SELENATE ION | O4 Se | 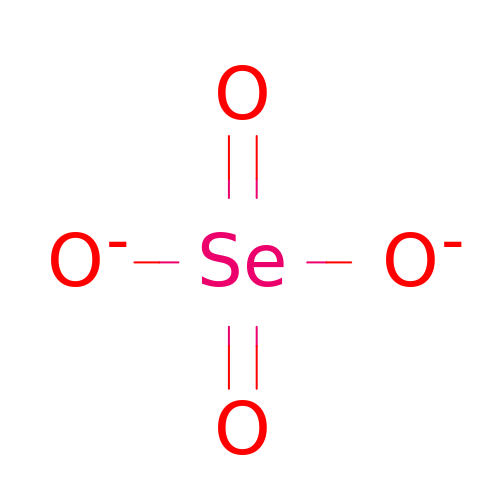QYHFIVBSNOWOCQ-UHFFFAOYSA-L> MGSRMITNEQDLKMFLLSKGASKEVIASIISRYPRAITRTPENLSKRWDLWRKIVTSDLEIVNILERSPESFFRSNNNLNLENNIKFLYSVGLTRKCLCRLLTNAPRTFSNSLDLNKQMVEFLQAAGLSLGHNDPADFVRKIIFKNPFILIQSTKRVKANIEFLRSTFNLNSEELLVLICGPGAEILDLSNDY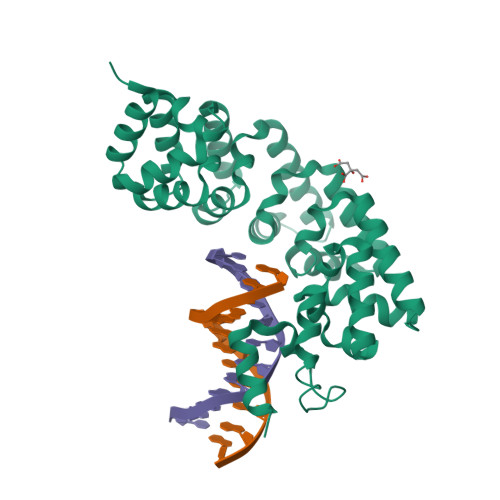ARRSYANIKEKLFSLGCTEEEVQKFVLSYPDVIFLAEKKFNDKIDCLMEENISISQIIENPRVLDSSISTLKSRIKELVNAGCNLSTLNITLLSWSKKRYEAKLKKLSRFAHHHHHH N-[(S)-({[(benzyloxy)carbonyl]amino}methyl)(hydroxy)phosphoryl]-L-leucyl-3-methyl-L-valine 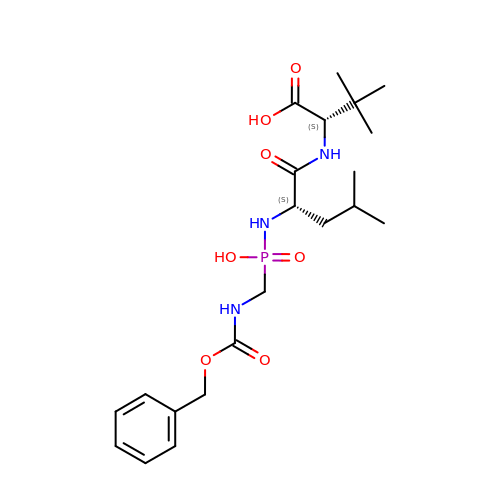| C21 H34 N3 O7 P | UVHGRCZPFAMOFG-DLBZAZTESA-N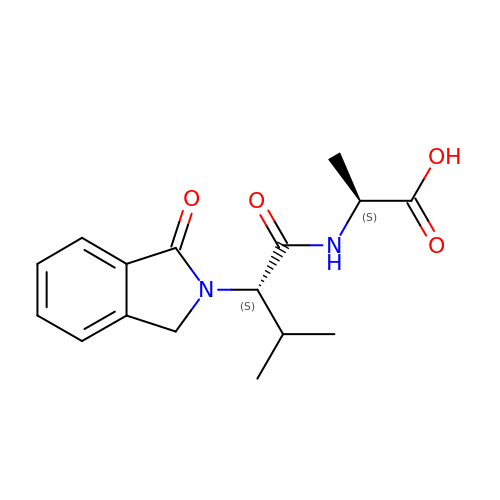(2~{S})-2-[[(2~{S})-3-methyl-2-(3-oxidanylidene-1~{H}-isoindol-2-yl)butanoyl]amino]propanoic acid | C16 H20 N2 O4 | ZLJCDMXBPPBVSF-GWCFXTLKSA-N>[60x]MYFFSVDPRN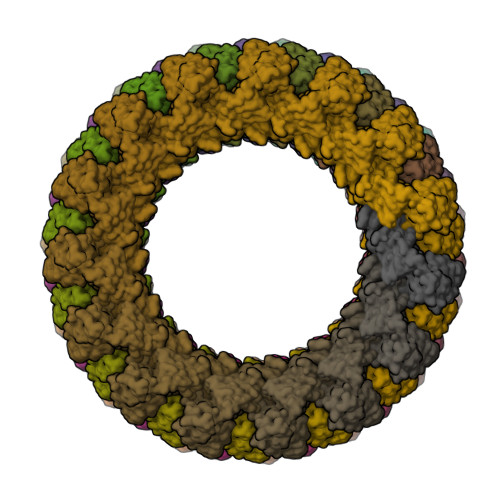GASKSGDVCGSCCCESISARPGEVNGVMVSYAAWSAPLRGHGLTNKTTFEIDGVSVTPPKVSNAFGRTKVGVVFEGTLSDLFPNPEGEQVEYEISELNGPSNGVVELGANGAFTYTPGALFTGVDRFWFSINGNIGEYVISVDPTTSELPQPPFTTPVYVPAARRSVDPRTHVLKFVLGVSPAAIPGDVYRLTVRQVAIDCDGNEFVHISCYDISIGSCG Sister chromatid cohesion is mediated by cohesin, whose Smc1, Smc3, and kleisin (Scc1) subunits form a ring structure that entraps sister DNAs. The ring is opened either by separase, which cleaves Scc1 during anaphase, or by a releasing activity involving Wapl, Scc3, and Pds5, which bind to Scc1 and open its interface with Smc3. We present crystal structures of Pds5 from the yeast L. thermotolerans in the presence and absence of the conserved Scc1 region that interacts with Pds5. Thus, Pds5 can be considered the gatekeeper of the cohesin ring.

We expressed Pds5 from Lachancea thermotolerans (Lt) in E. coli and determined its structure at 3.2 Å resolution (Experimental Procedures). LtPds5 is 47% identical in sequence to Saccharomyces cerevisiae (Sc) Pds5. The large molecule is exclusively alpha helical, composed of a large number of HEAT-like repeats and helical extensions/additions that deviate from the HEAT repeat pattern. The HEAT repeat pattern leads to a linear path from the N terminus to the C terminus, separating them by more than 100 Å. Deviations from the HEAT repeat pattern create a nose and extension domain, as well as a very pronounced hook, bending back so that the most C-terminal portion of Pds5 contacts the middle section, which contains the most regular HEAT repeats and which we called the spine. Bending back the hook creates a small loop or ring with an inner diameter of approximately 10 Å. When we plotted sequence conservation among Pds5 homologs onto the Pds5 structure, several regions of potential functional interest became apparent. Extending along one edge of the spine, region II runs all the way to the N-terminal region at the top, where it ends with a large patch of conservation. This region includes a loop with consensus sequence APDAP (residues 116–120 in LtPds5). When comparing the structure of Pds5 with the other HEAT-repeat-containing subunit of cohesin, Scc3 (Hara et al., 2014, Roig et al., 2014), striking similarities appear: both proteins contain hook, spine, extension, and nose and, intriguingly, bind their corresponding conserved Scc1 sites between the spine and the hook, forming a closed ring, and possibly creating another case of topological entrapment in the system.

> XXXXXXXXXXXXXXXXXXXXXXXXXXXXXXXXDLRSLERYRADLIDRKILRNKDHGVRAFAACCLSDILRLYAPDAPYTDKELTEIFRLFLAQLKLLQEPENGYLTQQTYLINNLLEYRSIVILTDLPSSSQLVEELFNIFYSPTNSTIQGNMFTAIGGILGEVISECDSLPMSALKMVFNKFLSHKRAESLDGINYKKDPGFEISLIICQTYSNRLGRHFIKFYSEIMYEVLGESDIHEKGIASSAYKTLVKIGNLTSELWKYAPELVGSVTGLLYQLLCSDNELFRESATKCVSKMLGTHSLINFAVAHSDTYKIWLSKMADISPHVRQAWVSEIPSILMSRSDLSDDISKGLAKALIDSDHTVRLSAIQTFHEVPVKRLWECLPNAAVFAGLVHLTRETRRDLRDECIDAVARIYTESIESIPKTNENKEIWGVVETIPSACFNLYYINDLEINMKVDLLTFEKFLPLGLSNEEFVQRLLTLLQGFNEKAFSSFYAFNRRQDQMSTVLWKFIEFCEETNSQSPAASLSDTKLIKTVEWISSGFPSHLNVEQILLAFRELNDRRLYRLIKVAVAETSKHLTVRNAVSELFKRLEEPELFRKKNIKIESRFTRDNFSTVFRVLIYRAAPIIFNISNLPSFLNTSDSSNEDEKALKRQLIDNISIIKPGIFKDQVKNLVTIITEGETTGPGNTLSLAEAMRTVYKISKDKREHLDIEENTFFFQKLEDYAKEGNPLEAKYAIKLLGLAPNAAEYLSEVATAILPLDLKSKHFASNVLVLAEITKMQPQLLEKDSTEIVGLLIKDVLLSNDVVGDEDDQQAWFSDEDIYTGKADALSAKVFSLKLFANKIKVMAPDAHADEMTHAFTERTLKLFFYLVASGGELVSESNTDNYPTPANYQNKLRCCAGLHILKITKIASLSRFIKPQDISKLMNLVEDESLEVRSSFIGRLKDFLGDGSISIKFLPLVFFTAYEPDQALRTSTKMWINYTLSKENFRKGTFFERALPRLIHFIAHHPDVAEGLRLRETAFLTGLTTAIDYLVFYADSVLKASNLALLYYLAGRVRQYXXXXXXXXXXXXXXXXXXXXXXXXXXXXXXXXXXXXXXXXXXXXXXXXXXXXXXXXXXXXXXXXXXXXXXXXXXXXXXXXXXXXXXXXXXXXXXXXXXXXXXXXXXXXX3-[3-[(7-methyl-1,8-naphthyridin-2-yl)carbamoyloxy]propylamino]propyl 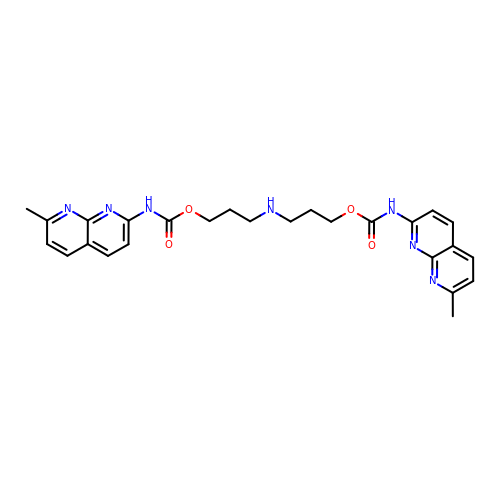~{N}-(7-methyl-1,8-naphthyridin-2-yl)carbamate | C26 H29 N7 O4 | RLXLNYXAIXVZCE-UHFFFAOYSA-N> GICKSSDCIKSAARLIQNMDATTEPCTDFFKYACGGWLKR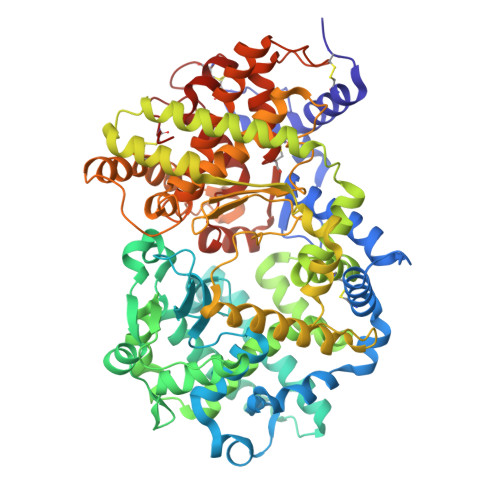NVIPETSSRYGNFDILRDELEVVLKDVLQEPKTEDIVAVQKAKALYRSCINESAIDSRGGEPLLKLLPDIYGWPVATENWEQKYGASWTAEKAIAQLNSKYGKKVLINLFVGTDDKNSVNHVIHIDQPRLGLPSRDYYECTGIYKEACTAYVDFMISVARLIRQEERLPIDENQLALEMNKVMELEKEIANATAKPEDRNDPMLLYNKMTLAQIQNNFSLEINGKPFSWLNFTNEIMSTVNISITNEEDVVVYAPEYLTKLKPILTKYSARDLQNLMSWRFIMDLVSSLSRTYKESRNAFRKALYGTTSETATWRRCANYVNGNMENAVGRLYVEAAFAGESKHVVEDLIAQIREVFIQTLDDLTWMDAETKKRAEEKALAIKERIGYPDDIVSNDNKLNNEYLELNYKEDEYFENIIQNLKFSQSKQLKKLREKVDKDEWISGAAVVNAFYSSGRNQIVFPAGILQPPFFSAQQSNSLNYGGIGMVIGHDITHGFDDNGRNFNKDGDLVDWWTQQSASNFKEQSQCMVYQYGNFSWDLAGGQHLNGINTLGENIADNGGLGQAYRAYQNYIKKNGEEKLLPGLDLNHKQLFFLNFAQVWCGTYRPEYAVNSIKTDVHSPGNFRIIGTLQNSAEFSEAFHCRKNSYMNPEKKCRVW> MALVDGFLELERSSGKLEWSAILQKMASDLGFSKILFGLLPKDSQDYENAFIVGNYPAAWREHYDRAGYARVDPTVSHCTQS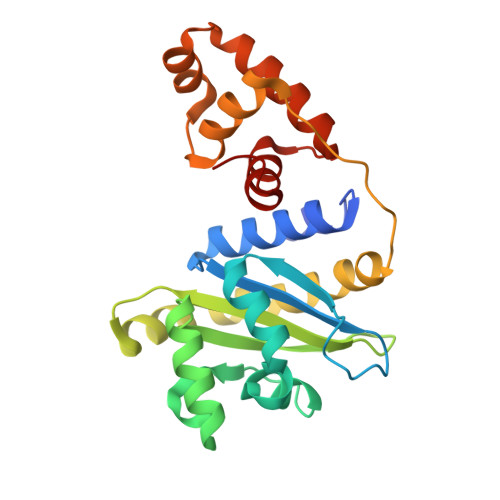VLPIFWEPSIYQTRKQHEFFEEASAAGLVYGLTMPLHGARGELGALSLSVEAENRAEANRFMESVLPTLWMLKDYALQSGAGLAFEHPVSKPVVLTSREKEVLQWCAIGKTSWEISVICNCSEANVNFHMGNIRRKFGVTSRRVAAIMAVNLGLITL>[8x]MMGRGKLILIEGLDRTGKTTQCNILYKKLQPNCKLLKFPERSTRIGGLINEYLTDDSFQLSDQAIHLLFS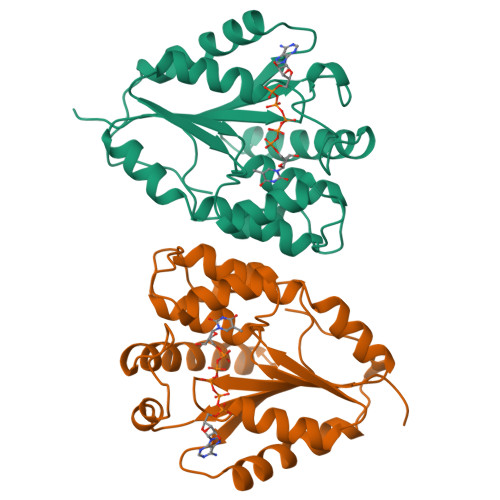ANRWEIVDKIKKDLLEGKNIVMDRYVYSGVAYSAAKGTNGMDLDWCLQPDVGLLKPDLTLFLSTQDVDNNAEKSGFGDERYETVKFQEKVKQTFMKLLDKEIRKGDESITIVDVTNKGIQEVEALIWQIVEPVLSTHIDHDKFSFF>MTDHARGTLPEIRRGRIYRDVYHKRVDEEPVDRTADLERARLGDDGLDFQDDAAQARAFAQGVFLLEIPEWLDLSAGDRFARQFFQGTGVEPYGKYRDLSSEHFGDELLGYHSRVDQLEQFLLERRFWGEVYPSEIATLGEHLTLLSHRVLRSVLASAGIPEEDWHRASGGCSETNGSYHLTFNHYRSAHQDIGLSSHKDDGFITVLRTTAQGLEVNRDDVWEKVPVDPACFVVNFGLSMEILTSACVTPLSAIMHRVSHQNFDRSSFGHFSSSRCLPGADDGIYRYLPSAGLERVCGSRELI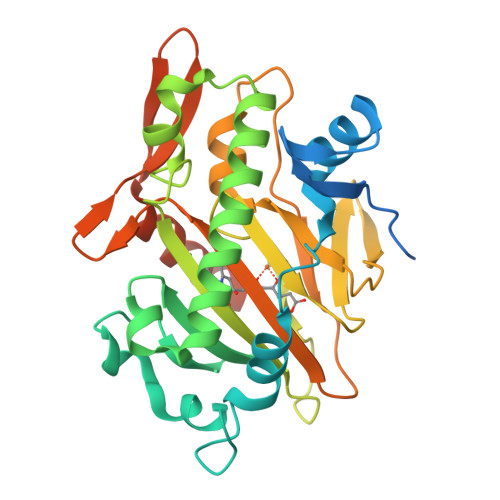EENDHEIYMGTEGQGLEHHHHHHHH[3x]> MN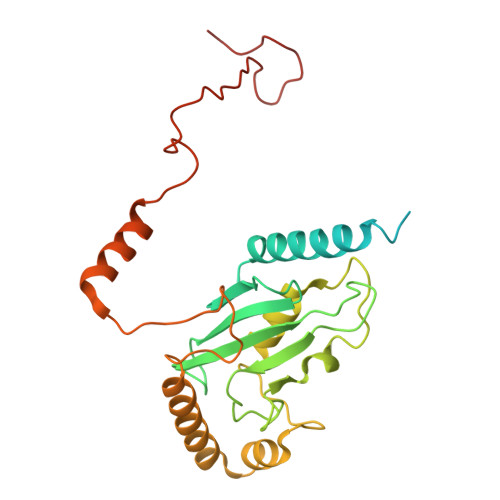PFWSMSTSSVRKRSEGEEKTLTGDVKTSPPRTAPKKQLPSIPKNALPITKPTSPAPAAQSTNGTHASYGPFYLEYSLLAEFTLVVKQKLPGVYVQPSYRSALMWFGVIFIRHGLYQDGVFKFTVYIPDNYPDGDCPRLVFDIPVFHPLVDPTSGELDVKRAFAKWRRNHNHIWQVLMYARRVFYKIDTASPLNPEAAVLYEKDIQLFKSKVVDSVKVCTARLFDQPKIEDPYAISFSPWNPSVHDEAREKMLTQKKPEEQHNKSVHVAGLSWVKPGSVQPFSKEEKTVAT> STTSSRVDDHDSEEICLDHLCKGCPLNGSCSKVHFHLPYRWQMLIGKTWTDFEHMETIEKGYCNPGIHLCSVGSYTINFRVMSCDSFPIRRLSTPSSVTKPANSVF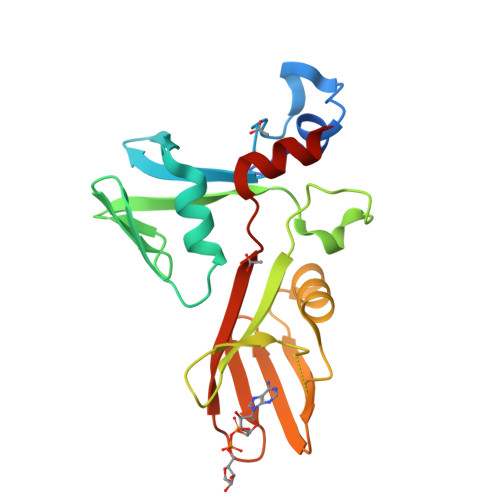TTKWIWYWKNESGTWIQYGEEKDKRKNSNVDSSYLESLYQSCPRGVVPFQAGSRNYELSFQGMIQTNIASKTQKDVIRRPTFVPQWYVQQMKRGPD> ETGTTVPRVAFYAGLKNPHEGYEVLKFDDVVTNLGNNYDAASGKFTCNIPGTYFFTYHVLMRGGDGTSMWAD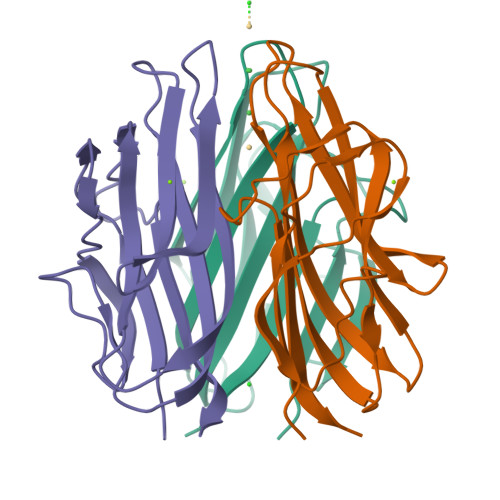LCKNGQVRASAIAQDADQNYDYASNSVILHLDAGDEVFIKLDGGKAHGGNSNKYSTFSGFIIYSDGTKHHHHHH>AGHMRLTMHVPDEDMLSPLGALRLDGHFSFHDVSAMARDFGNQCSFLPAAVLHPGSVSDIAATVRHVFSLGEGSPLTVAARGHGHSLMGQSQAAQGIVVRMESLRGARLQVHDGFVDAPGGELWINVLRETLKHGLAPKSWTDYLHLTVGGTLSNAGVSGQAFRHGPQVSNVNQLEIVTGRGDVVTCSPEDNSDLFYAALGGLGQFGIITRARIALEPAPEMVRWIRVLYSDFESFTEDQEMLIMAENSFDYIEGFVIINRTGILNNWRASFKPQDPVQAS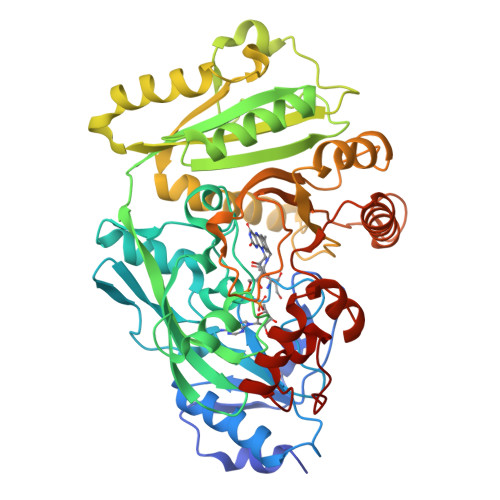HFQSDGRVLYCLELTKNFNSGDTDTMEQEVAVLLSRLRFIQSTLFHTDVTYLEFLDRVHTSELKLRAQSLWEVPHPWLNLLIPRSSIRRFATEVFGRILKDSNNGPILLYPVNKSKWDNKTSVVIPDEEIFYLVGFLSSAPSLSGHGSIAHAMSLNSQIVEFCEEADIGMKQYLAHYTTQEQWKTHFGARWETFERRKHRYDPLAILAPGQRIFPKASLP[4x]> SSESTTFIVDVSPSMMKNNNVSKSMAYLEYTLLNKSKKSRKTDWISCYLANCPVSENSQEIPNVFQIQSFLAPVTTTATIGFIKRLKQYCDQHSHDSSNEGLQSMIQCLLVVSLDIKQQFQARKILKQIVVFTDNLDDLDITDEEIDLLTEELSTRIILIDCGKDTQEERKKSNWLKLVEAIPNSRIYNMNELLVEITSPATSVVKPVRVFSGELRLGADILSTQTSNPSGSMQDENCLCIKVEAFPATKAVSGLNR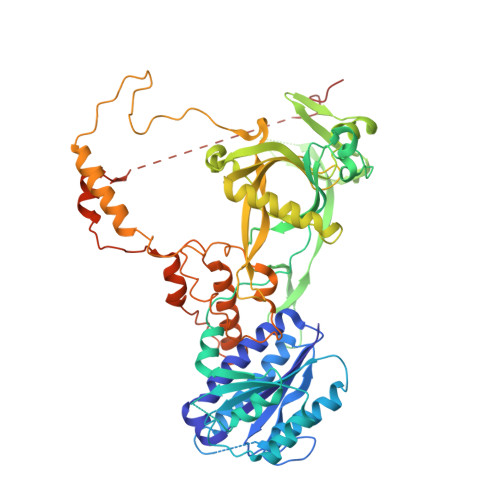KTAVEVEDSQKKERYVGVKSIIEYEIHNEGNKKNVSEDDQSGSSYIPVTISKDSVTKAYRYGADYVVLPSVLVDQTVYESFPGLDLRGFLNREALPRYFLTSESSFITADTRLGCQSDLMAFSALVDVMLENRKIAVARYVSKKDSEVNMCALCPVLIEHSNINSEKKFVKSLTLCRLPFAEDERVTDFPKLLDRTTTSGVPLKKETDGHQIDELMEQFVDSMDTDELPEIPLGNYYQPIGEVTTDTTLPLPSLNKDQEENKKDPLRIPTVFVYRQQQVLLEWIHQLMINDSREFEIPELPDSLKNKISPYTHKKFDSTKLVEVLGIKKVDKLKLDSELKTELEREKIPDLETLLKRGEQHSRGSPNNSNN> DEQPEPRTRRRAYLWCKEFLPGAWRGLREDEFHISVIRGGLSNMLFQCSLPDTTATLGDEPRKVLLRLYGAILQMRSCNKEGSEQAQKENEFQGAEAMVLESVMFAILAERSLGPKLYGIFPQGRLEQFIPSRRLDTEELSLPDISAEIA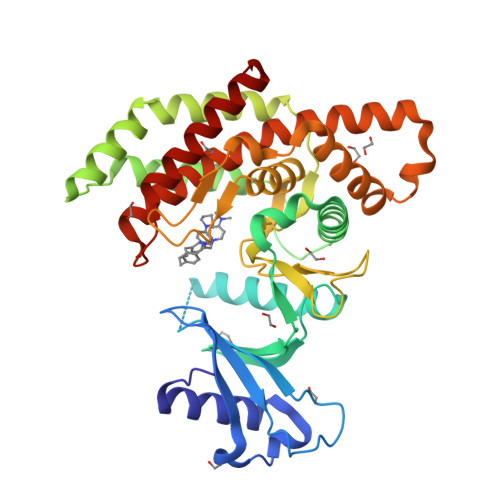EKMATFHGMKMPFNKEPKWLFGTMEKYLKEVLRIKFTEESRIKKLHKLLSYNLPLELENLRSLLESTPSPVVFCHNDCQEGNILLLEGRENSEKQKLMLIDFEYSSYNYRGFDIGNHFCEWMYDYSYEKYPFFRANIRKYPTKKQQLHFISSYLPAFQNDFENLSTEEKSIIKEEMLLEVNRFALASHFLWGLWSIVQAKISSIEFGYMDYAQARFDAYFHQKRKLGV> AQFKEGEHYQVLKTPASSSPVVSEFFSFYCPHCNTFEPIIAQLKQQLPEGAKFQKNHVSFMGGNMGQAMSKAYATMIALEVEDKMVPVMFNRIHTLRKPPKDEQELRQIFLDEGIDAAKFDAAYNGFAVDSMVRRFDKQFQDSGLTGVPAVVVNNRYLVQGQSAKSLDEYFDLVNYLLTLK

DsbA enzymes catalyze oxidative folding of proteins that are secreted into the periplasm of Gram‐negative bacteria, and they are indispensable for the virulence of human pathogens such as Vibrio cholerae and Escherichia coli. DsbA enzymes retain a conserved tertiary structure, comprising a classical thioredoxin (TRX) domain with an inserted α‐helical domain. The TRX domain contains a pair of redox‐active cysteine residues in a CXXC motif located adjacent to a conserved cis‐proline residue. These features contribute to a hydrophobic patch of residues located in a surface groove of DsbA that is required for substrate recognition.

To identify the structural details of the interaction between TC and DsbA, we solved the crystal structures of TC in complex with oxidized EcDsbA and VcDsbA using molecular replacement at resolutions of 1.79 Å and 1.74 Å, respectively. TC also binds to the hydrophobic groove of VcDsbA but adopts a different binding pose compared to the complex with EcDsbA. The binding contributes to a buried SASA of 401 Å2, which is similar to that of the EcDsbA‐TC complex. The binding of TC does not cause major conformational change of VcDsbA. The hydrophobic groove of VcDsbA is truncated and flatter than the groove of EcDsbA as a result of a three‐residue deletion in loop L3 and a four‐residue deletion in helix H7. The VcDsbA‐TC complex shows that TC binds only to the right‐hand side of the VcDsbA groove where it makes hydrophobic contacts with A164, K165, S166 and L167 of loop L3. This results in the polar end of TC binding directly under H32 of the active site. Close inspection of the crystal structure also showed that TC makes additional hydrophobic contacts with R107 and D121 of a symmetry‐related molecule in the crystal lattice. Residues Q162, A164, K165, L167 and Y170 of VcDsbA, which are strongly perturbed upon addition of TC in the HSQC spectra, are all located within 5 Å of TC in the crystal structure.>[2x]MSSGNAKIGHPAPSFKATAVMPDGQFKDISLSDYK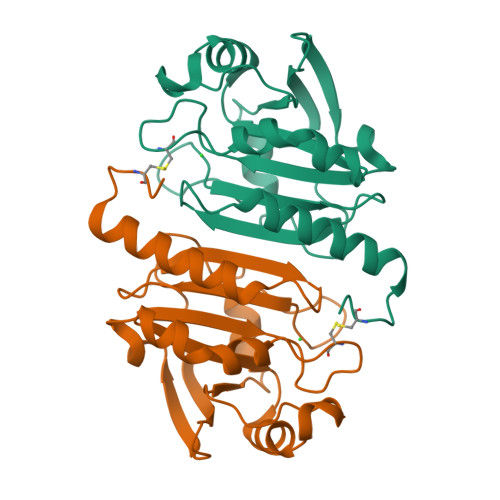GKYVVFFFYPLDFTFVCPTEIIAFSDRAEEFKKLNCQVIGASVDSHFSHLAWINTPKKQGGLGPMNIPLVSDPKRTIAQDYGVLKADEGISFRGLFIIDDKGILRQITINDLPVGRSVDEILRLVQAFQFTDKHGEVCPAGWKPGSDTIKPDVNKSKEYFSKQK>[4x]VHYGLKGITCVETSISHIDGEKGRLIYRGHHAKDI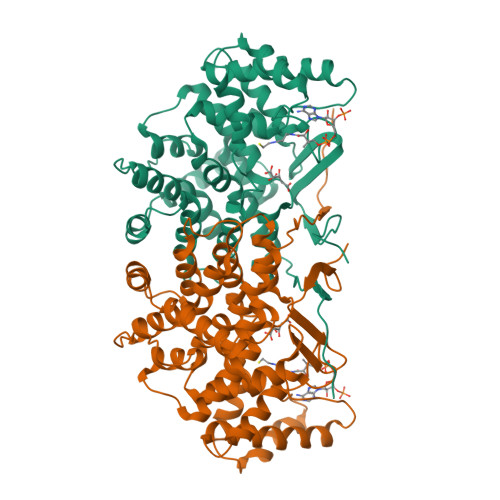ALNHSFEEAAYLILFGKLPSTEELQVFKDKLAAERNLPEHIERLIQSLPNNMDDMSVLRTVVSALGENTYTFHPKTEEAIRLIAITPSIIAYRKRWTRGEQAIAPSSQYGHVENYYYMLTGEQPSEAKKKALETYMILATEHGMNASTFSARVTLSTESDLVSAVTAALGTMKGPLHGGAPSAVTKMLEDIGEKEHAEAYLKEKLEKGERLMGFGHRVYKTKDPRAEALRQKAEEVAGNDRDLDLALHVEAEAIRLLEIYKPGRKLYTNVEFYAAAVMRAIDFDDELFTPTFSASRMVGWCAHVLEQAENNMIFRPSAQYTGAIPEEV> SGHKPVPCGWERVVKQRLSGKTAGKFDVYFISPQGLKFRSKRSLANYLLKNGETFLKPEDFNFTVL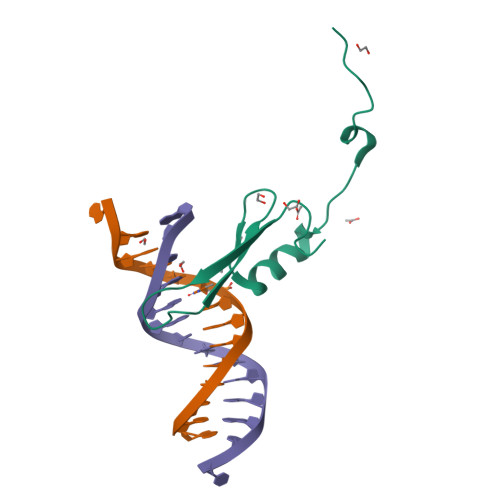PKG> GAACGACACAGA;> CGACGACTC;> TCTTCG;> TCGAGTCGGTGTCGT

In this work, we exhaustively probe the ability of all 36 immobile HJ sequences to form DNA crystals in two different designed systems. Three separate self-assembling DNA crystal systems are described in this report: the “4 × 5” and “4 × 6” designs (collectively referred to as the 4 × N systems), and a third construct with a “scrambled” sequence variant of the 4 × 6 lattices. Self-assembly was mediated by three constituent oligonucleotides: (S1) containing four sequence repeats of either 5 or 6 bases; (S2) composed of 21 bases containing complementary regions to both (S1); and (S3) which forms the second junction crossover. The HJ serves as the fundamental component at the core of each unit, and the ultimate assembly of the full lattice is facilitated by the complementary 2-base sticky ends that tail each duplex.

To investigate this possibility, we designed “scrambled” sequences with targeted base substitutions, while maintaining GC content, along each “stem”. Contrary to the buffer preference observed with the native P32 crystals, the scrambled systems exhibited an exclusive preference towards low salt buffers, much like the native R3 crystals. Remarkably, only J1 and J2 retained the P32 symmetry, with all others yielding an R3 lattice. There appeared to be only a marginal difference in the average cell lengths in the R3 scramble crystals (a = b = 113.04 c = 51.10) relative to the native 4 × 6 sequences: the a, b axis trended ~2 Å shorter and c ~1.3 Å longer, whereas in the J1 and J2 cases, the crystals were in good agreement with the original 4 × 6 motif. The average angles of the R3 and P32 crystals were 61.00° (σ = 1.21) and 58.05° (σ = 1.39), respectively. Another major observation is the importance of stem region sequences outside the HJ, given that this sequence can control crystal symmetry and lattice architecture, and improve resolution in non-obvious ways. However, in the majority of the crystal structures reported here, the cacodylate anion indeed fits best into the electron density map of our X-ray structures, due to the presence of sodium cacodylate in the crystallization solution.>RHMRIAVIGGGSSYTPELVKGLLDISEDVRIDEVIFYDIDEEKQKIVVDFVKRLVKDRFKVLISDTFEGAVVDAKYVIFQFRPGGLKGRENDEGIPLKYGLIGQETTGVGGFSAALRAFPIVEEYVDTVRKTSNATIVNFTNPSGHITEFVRNYLEYEKFIGLCNVPINFIREIAEMFSARLEDVFLKYYGLNHLSFIEKVFVKGEDVTEKVFENLKLKLSNIPDEDFPTWFYDSVRLIVNPYLRYYLMEKKMFKKISTHELRAREVMKIEKELFEKYRTAVEIPEELTKRGGSMYSTA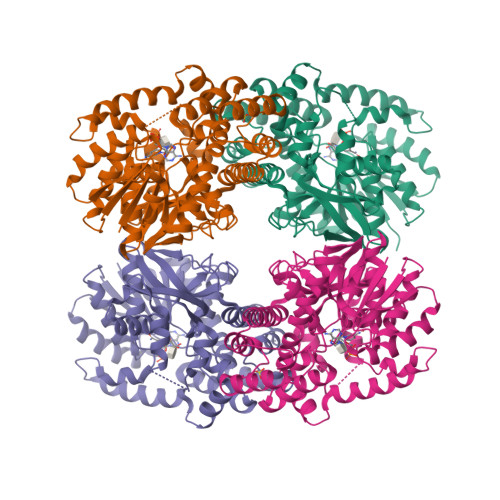AAHLIRDLETDEGKIHIVNTRNNGSIENLPDDYVLEIPCYVRSGRVHTLSQGKGDHFALSFIHAVKMYERLTIEAYLKRSKKLALKALLSHPLGPDVEDAKDLLEEILEANREYVKLG[8x]> MTLQKDKVIKWVRFTPPQVLAIGFFLTIIIGAVLLMLPISTTKPLSWIDALFTAASATTVTGLAVVDTGTQFTVFGQTVIMGLIQIGGLGFMTFAVLIVMILGKKIGLKERMLVQEALNQPTIGGVIGLVKVLFLFSISIELIAALIL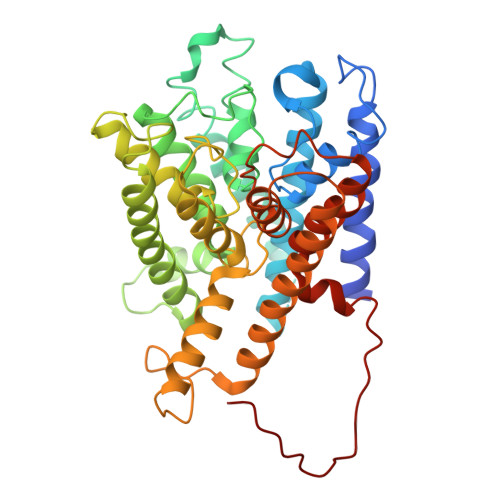SIRLVPQYGWSSGLFASLFHAISAFNNAGFSLWPDNLMSYVGDPTVNLVITFLFITGGIGFTVLFDVMKNRRFKTFSLHTKLMLTGTLMLNAIAMLTVFILEYSNPGTLGHLHIVDKLWASYFQAVTPRTAGFNSLDFGSMREGTIVFTLLLMFIGAGSASTASGIKLTTFIVILTSVIAYLRGKKETVIFRRSIKYPIIIKALAVSVTSLFIVFLGIFALTITEQAPFLQIVFETFSAFGTVGLTMGLTPELTTAGKCIIIVIMFIGRIGPLTFVFSFAKTEQSNIRYPDGEVFTG> MKPTIPPDDSDTAGKQVEVEKENETIQELMIALQIHSGYTNISYTI;> MSLILDDIILSLTNANERTPPQALKTTLSLLYEKSKQYGLSSPQLQALVRLLCETSIIDTVTKVYIVENCFLPDGYLTKELLLEIINHLGTPTVFSRYRIQTPPVLQSALCKWLVHVYFLFPVHSEREHNISSSIWLHLWQFSFLQKWITPLVIWQATTPVDVKPWKLSIIKRCAMHPGYRDAPGSATLILQRFQCLVGASSQITESIITINCNRKTLKSHRNLKLDAHFLSILKRILSRAHPANENLYFQ;> MKKQDHAHIRTRKARNKELWDSLADFLKGYLVPNLDDNDESIDSLTNEVMLLMKRLIEHDLNLTLNDFSSKTIPIYRLLLRANIITVIEGSTNPGTKYIKLIDFNETSLT;> MSTPRKAAGNNENTEVSEIRTPFRERALEEQRLKDEVLIRNTPGYRKLLSASTKSHDILNKDPNEVRSFLQDLSQVLARKSQGNDTTTNKTQARNLIDELAYEESQPEENELLRSRSEKLTDNNIGNETQPDYTSLSQTVFAKLQERDKGLKSRKIDPIIIQDVPTTGHEDELTVHSPDKANSISMEVLRTSPSIGMDQVDEPPVRDPVPISITQQEEPLSEDLPSDDKEETEEAENEDYSFENTSDENLDDIGNDPIRLNVPAVRRSSIKPLQIMDLKHLTRQFLNENRIILPKQTWSTIQEESLNIMDFLKQKIGTLQKQELVDSFIDMGIINNVDDMFELAHELLPLELQSRIESYLFENLYFQ;> MDTEALANYLLRQLSLDAEENKLEDLLQRQNEDQESSQEYNKKLLLACGFQAILRKILLDARTRATAEGLREVYPYHIEAATQAFLDSQ

Kinetochores are large multi-subunit complexes that attach centromeric chromatin to microtubules of the mitotic spindle, enabling sister chromatid segregation in mitosis. The inner kinetochore constitutive centromere associated network (CCAN) complex assembles onto the centromere-specific Cenp-A nucleosome (Cenp-ANuc), thereby coupling the centromere to the microtubule-binding outer kinetochore. CCAN is a conserved 14–16 subunit complex composed of discrete modules. Cenp-TW interacts directly with Cenp-HIKM to form a six-subunit complex (Cenp-HIKM-TW) in vertebrates, and a five-subunit complex (Cenp-HIK-TW) in budding yeast.

Here, we determined the crystal structure of the Saccharomyces cerevisiae Cenp-HIKHead-TW sub-module, revealing how Cenp-HIK and Cenp-TW interact at the conserved Cenp-HIKHead–Cenp-TW interface. The structure of the S. cerevisiae Cenp-HIKHead sub-module at 2.9 Å resolution is essentially identical to its counterpart in the thermophilic yeast. Cenp-HIKHead is assembled from the N-terminus of Cenp-IHead (residues 1–241) and the C-termini of Cenp-H (residues 147–181, Cenp-HHead) and Cenp-K (residues 136–237, Cenp-KHead). Although we crystallized a complex of Cenp-HIKHead-Cenp-TW using the full-length Cenp-T subunit, in our structure the N-terminal 268 residues are disordered, consistent with disorder predictions, with only the HFD and HFE being visible. The crystal structure of the Cenp-HIKHead-TW sub-module reveals that the major contacts between Cenp-HIKHead and Cenp-TW involve Cenp-IHead and Cenp-KHead of Cenp-HIK and Cenp-T of Cenp-TW, with Cenp-HHead and Cenp-W making minor contributions. In interface 1, the C-terminal anti-parallel α-helices (H4 and H5) of the HFE of Cenp-T combine with H3 of Cenp-K to create a compact three helix bundle. Interface 1 is dominated by a network of electrostatic interactions involving Arg206 and Arg210 of Cenp-K and Asp338, Glu357 and Ser354 of Cenp-T. In interface 2, the conserved L5 loop (residues 177–182) of Cenp-IHead inserts into a cavity within the Cenp-TW dimer formed by the interface of H1 of the Cenp-T HFD, turn connecting H4-H5 of the Cenp-T HFE, and N-terminus of Cenp-W. His177Cenp-I in the L5 loop, a highly conserved residue, makes an important contribution by providing a C-terminal helix cap to H4 of Cenp-T. We fitted the Cenp-HIKHead-TW sub-module to the previously determined cryo-EM map of the S. cerevisiae CCAN–Cenp-ANuc complex. This showed that the HEAT repeat domain of Cenp-IHead and C-terminal HFD of Cenp-T of the Cenp-HIKHead-TW sub-module interact with the nucleosome DNA gyre at a site close to the Cenp-ANuc dyad axis.> GPLGSMASITQLFDDLCEALLPAAKTHLGQRSVNRKRAKRSLKKVAYNALFTNLFQDETQQLQPDMSKLPARNKILMLSFDLRVGGLGPKADRLEELVEELEAAPCCPLLEVGSVLDLLVQLAG;> GPHMASSSGAGAAAAAAAANLNAVRETMDVLLEIS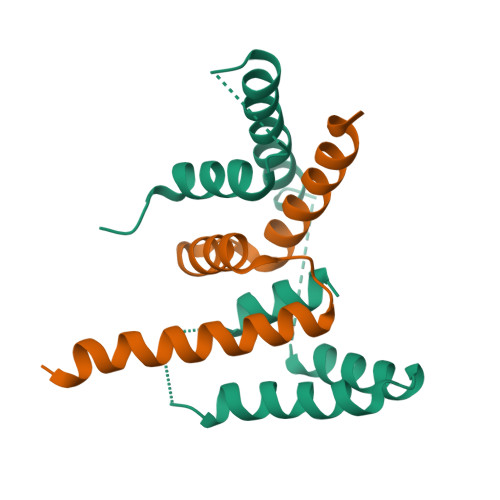RILNTGLDMETLSICVRLCEQGINPEALSSVIKELRKATEALKAAENMTS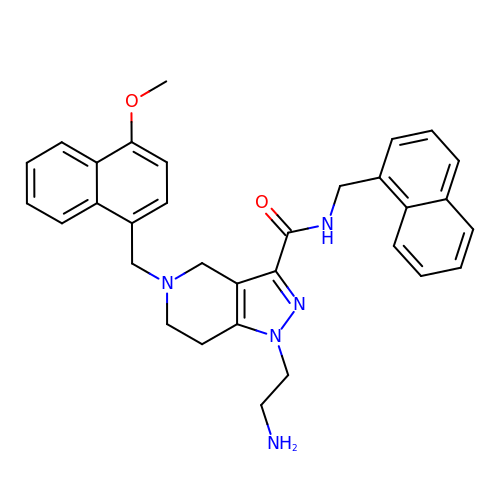1-(2-azanylethyl)-5-[(4-methoxynaphthalen-1-yl)methyl]-~{N}-(naphthalen-1-ylmethyl)-6,7-dihydro-4~{H}-pyrazolo[4,3-c]pyridine-3-carboxamide | C32 H33 N5 O2 | WADXPVUOGGMXPD-UHFFFAOYSA-N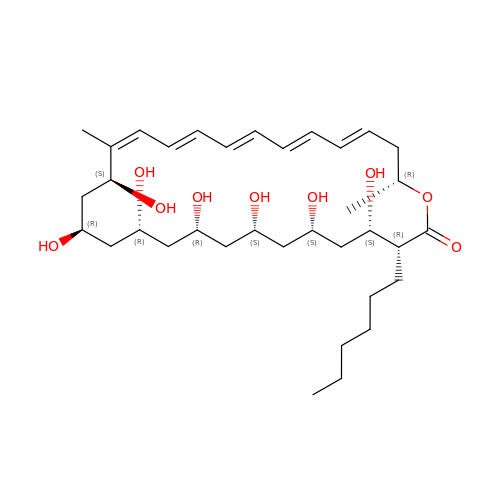(3R,4S,6S,8S,10R,12R,14R,16S,17E,19E,21E,23E,25E,28R)-3-hexyl-4,6,8,10,12,14,16-heptahydroxy-17,28-dimethyloxacyclooctacosa-17,19,21,23,25-pentaen-2-one | C35 H58 O9 | FODXYXCKUOAJAV-XHDOTJGXSA-N At the cytoplasmic face of the NPC, Nxf1•Nxt1-bound mRNPs encounter the cytoplasmic filament nucleoporins Gle1, Nup42, and Nup214, which specifically activate the DEAD-box helicase DDX19 to remove Nxf1•Nxt1 from the mRNP8. DDX19 is a member of the DEAD-box helicase family, which are RNA-dependent ATPases composed of two RecA domains (referred to as DDX19NTD and DDX19CTD throughout the text). Gle1CTD plays an important organizational role by providing spatially separated binding sites for Nup42GBM and the DEAD-box helicase DDX19/scDbp5. A comprehensive structure-function analysis of DDX19 indicates that binding of Gle1CTD•Nup42GBM induces a conformational change in DDX19, thereby stimulating its ATPase activity.

To evaluate whether the mode of interaction observed for S. cerevisiae Gle1CTD•Nup42GBM was conserved in other eukaryotes, we determined the crystal structures of human Gle1CTD•Nup42GBM at 2.8 Å resolution and of C. thermophilum Gle1CTD•Nup42GBM in the presence and absence of IP6 at 2.17 and 2.65 Å resolution, respectively. The overall structure of Gle1CTD is conserved between fungi and humans, with minor differences resulting from small insertions or different loop sizes. Both human and C. thermophilum Nup42GBM adopt the same fold as S. cerevisiae Nup42GBM and recognize the same surface on Gle1CTD, with the critical hydrophobic residues nearly universally conserved. Similarly, C. thermophilum Gle1CTD•Nup42GBM undergoes minimal conformational changes upon IP6 binding, which are mostly limited to a loop directly adjacent to the IP6 pocket. The interaction between C. thermophilum Gle1CTD•Nup42GBM and Dbp5 also required IP6, consistent with the evolutionary conservation of the IP6 binding residues among fungi. Strikingly, the Gle1CTD•Nup42GBM interaction mechanism is virtually identical in species separated by more than a billion years of evolution.

>[4x]GPHMRYVEIHRNLKGLRKYMAEQAKTNLKLKQRMGDMRREIRKSVGQLTTGGMAANKDKQQKIKSILTEALSNQVESALVDPNNFVVEPRKPVEGATNNDPLLPSIFVYLINIFAKAAISQFINEAGARPETADPVGICVAAILSEPDFLWRGASLIDILIAKFRIVCPVLFGYRGSEKTEQGRQRLGWWKESGQWISEQQHMDRMTGLGAGFAAISLRKFALSKKQNPYPPRFYWMAMAKIVNTPPAEISNTQCVVLKAMVQNYEAKFIEFYGSAAIAALRTALIDFPARAPHKSAAVNSLEVLAQMLKRDTGLDLG;>[4x]GPHMGSPEFDGTLVRIWMPDGAPAYTADTEAEDPKVYEDEGVKRQWQSFLEKGRFEGGMPEVPPRREWCVWDF7,8-dimethoxy-3-methyl-1~{H}-3-benzazepin-2-one | C13 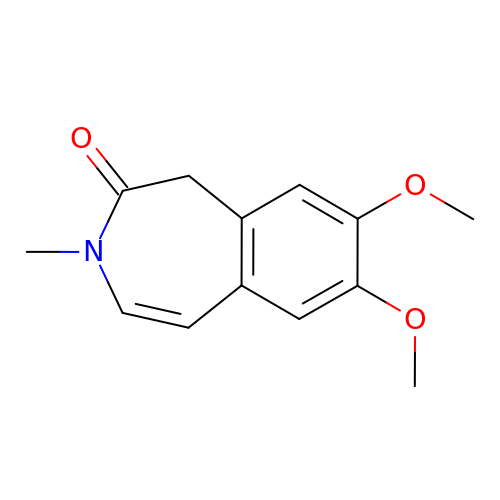H15 N O3 | SNBSBSFGIKHBLT-UHFFFAOYSA-N Dna2 has nuclease and helicase activities and plays key roles in maintaining genomic integrity. It is involved in the nucleolytic processing of 5’ flaps during Okazaki fragment maturation, of DNA double-strand breaks (DSBs) during homologous-recombination mediated repair, and of stalled replication forks in the intra-S-phase checkpoint. Dna2 contains a PD-(D/E)XK superfamily nuclease motif and a 5’ to 3’ helicase domain. It is a ssDNA endonuclease that requires a free end for cleavage, and does not cleave dsDNA, single-stranded gaps, D-loops or RNA.

The Dna2-ssDNA structure shows that the active site and most of the DNA-binding sites are enclosed in a narrow tunnel, necessitating the threading of the DNA through a tunnel end to access the DNA binding sites. The structure explains why the nuclease activity of Dna2 requires the ssDNA to have a free end. The active site is embedded in a ∼10 Å wide portion of the tunnel, and the tunnel entrances leading to it are too narrow to accommodate dsDNA or a single-stranded loop of a gap substrate. DNA binds to Dna2 through both its phosphodiester and base groups. Dna2-phosphodiester interactions involve protein pockets that are rich in backbone amide and short-side chain hydroxyl groups.

>MEPLDELDLLLLEEDGGAEAVPRVELLRKKADALFPETVLSRGVDNRYLVLAVETSQNERGAEEKRLHVTASQDREHEVLCILRNGWSSVPVEPGDIVHLEGDCTSEPWIIDDDFGYFILYPDMMISGTSVASSIRCLRRAVLSETFRGSDPATRQMLIGTILHEVFQKAISESFAPERLQELALQTLREVRHLKEMYRLNLSQDEILCEVEEYLPSFSKWAEDFMRKGPSSEFPQMQLSLPSDGSNRSSPCNIEVVKSLDIEESIWSPRFGLKGKIAVTVGVKIHRDCKMKYKVMPLELKTGKESNSIEHRSQVVLYTLLSQERREDPEAGWLLYLKTGQMYPVPANHLDKRELLKLRNWLAASLLHRVSRAAPGEEARLSALPQIIEEEKTCKYCSQIGNCALYSRAVEEQGDDASIPEAMLSKIQEETRHLQLAHLKYFSLWCLMLTLESQSKDNRKTHQSIWLTPASELEESGNCVGNLVRTEPVSRVCDGQYLHNFQRKNGPMPATNLMAGDRIILSGEERKLFALSKGYVKKMNKAAVTCLLDRNLSTLPATTVFRLDREERHGDISTPLGNLSKLMESTDPSKRLRELIIDFREPQFIAYLSSVLPHDAKDTVANILKGLNKPQRQAMKRVLLSKDYTLIVGMPGTGKTTTICALVRILSACGFSVLLTSYTHSAVDNILLKLAKFKVGFLRLGQSHKVHPDIQKFTEEEICRSRSIASLAHLEELYNSHPIVATTCMGINHPIFSRKTFDFCIVDEASQISQPVCLGPLFFSRRFVLVGDHQQLPPLVVNREARALGMSESLFKRLERNESAVVQLTVQYRMNRKIMSLSNKLTYAGKLECGSDRVANAVLALPNLKDARLSLQLYADYSDSPWLAGVLEPDNPVCFLNTDKVPAPEQVENGGVSNVTEARLIVFLTSTFIKAGCSPSDIGVIAPYRQQLRIISDLLARSSVGMVEVNTVDKYQGRDKSLILVSFVRSNEDGTLGELLKDWRRLNVALTRAKHKLILLGSVSSLKRFPPLGTLFDHLNAEQLILDLPSREHESLSHIL[2x]(2R)-2-butylbutanedioic acid | C8 H14 O4 | 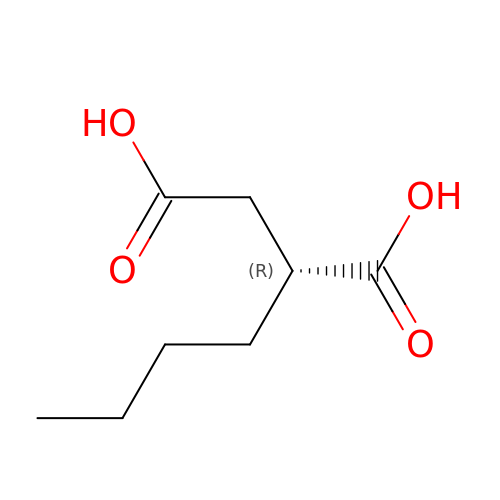WOPLHDNLGYOSPG-ZCFIWIBFSA-N>[3x]MKKSLIALTTALSFGLAAAQTAAPVSAPQVPALTDVPAGHWAKDAIDRLVSRGVILGYPDGTFRGTQNLTRYEAAIIIARLLDQMRDGETPAGMTAEDMTALQNAIQELAADLAALGVRVSDLEANAVSKDDFARLEARIEEVAAAGGEQGATEALQGQIDDLTARVDEYDALRADVDDNASSIAALNDLTVLLNQDILDLQDRVSAVEAAQADFVQRSDFDALGGRVTTVETRVETVNNSLTGRIAALERNAFSVKPSLTIGYSVSRTSRNFDVDRLFPLNADGTVANNAFTSGGIDTDTGAQRRDFGDFGNASDPVVAGAAGLYGFADGVSYTVYFTDGSTATFDGLNPADYKVPTGKVIDTTKGRNGFGFNNLARYKEGSTDIGISLGFDTSGQFSQVTSGTGGSLFSTAGRLQVNQIDLNFGLVTGLPSDAYVDTNGNGKKDDGEATGRGTYLGSGGTAAILRDPAGNVYRPVFFRFKNATTQFSVGNNPVIVTLGQQQKFYFSDYVFDNNYDGRGDGFTVTVDGSNVPVIGAWKPQIKGVYGSRSGLDGTAEAGYGVYYRGVRAQITPVGTLTAGIHYAQEGRDMFGAAQNTTSTPSDVTTYGADLHGKAFGVELHSEYATSRVRPNTANAAVQTSNAFYARVATRKDNLAFDL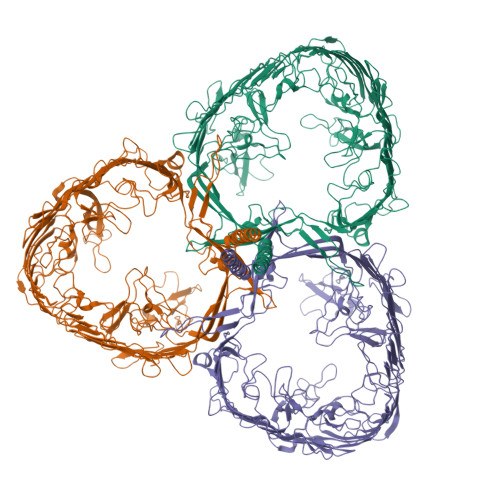NTPAAKFGNDTFGVSLYDLNYRKIDAGYNNVAGISEYGYGSYSRTSAQNIAYNPDTGVTAPFANLDRQAYTDANNDGTSDRNADGTVVATNTKIGQMGFGVKAAANLGPVAIGGYYDTSTGANGDNANRMTEAGGSAKVAYSIFSLRGTYNTLDSNRPQIYRDAAGTQIIGDAKVRRYAVQADVTPGLGLFVGAYYRDVNVNGVRSTTDRGLLGRGYLASSFEPGVGNNAYRTGLRCADNNFGTGTRDIDGVGGVLNPAVNLDQSRTATCFTSYGVEAGHAGDNANALVKDLFFRVGYSRVYVPTTATATTGDFSGSVTYGDARYDRKVGVANVRLAGSFSTTNTQLDSRPAGTRGAVGLIVRTDPLENVPFRPQFNGQVGYYTADNRVAAGNYNANATKYGAGVVLNDFLLPQTKIGVRYDGYMAQNRQYTPFDGDGTQGYFSDANNNRRTNLNGVYVEGAYQDLIFSYGTYTLSQKDLNGVEYGSGINNGQPARGQTFKISYKVNF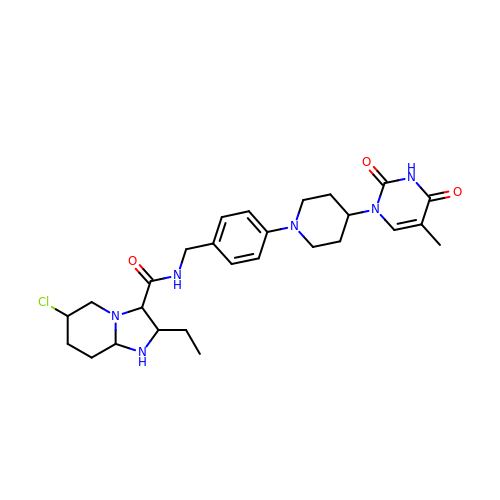2-ethyl-~{N}-[[4-[4-[5-methyl-2,4-bis(oxidanylidene)pyrimidin-1-yl]piperidin-1-yl]phenyl]methyl]-1,2,3,5,6,7,8,8~{a}-octahydroimidazo[1,2-a]pyridine-3-carboxamide | C27 H37 Cl N6 O3 | ZMLCAZKJSUZKPA-UHFFFAOYSA-N2-methoxy-5-nitro-phenol 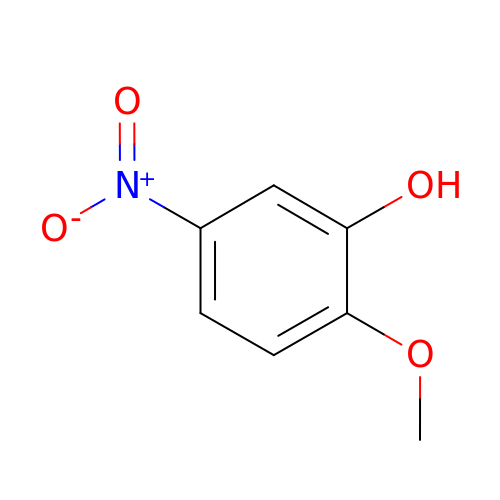| C7 H7 N O4 | KXKCTSZYNCDFFG-UHFFFAOYSA-N>SNAMWESKFVKEGLTFDDVLLVPAKSDVLPREVSVKTVLSESLQLNIPLISAGMDTVTEADMAIAMARQGGLGIIHKNMSIEQQAEQVDKVKRSGGLLVGAAVGVTADAMTRIDALVKASVDAIVLDTAHGHSQGVIDKVKEVRAKYPSLNIIAGNVATAEATKALIEAGANVVKVGIGPGSICTTRVVAGVGVPQLTAVYDCATEARKHGIPVIADGGIKYSGDMVKALAAGAHVVMLGSMFAGVAESPGETEIYQGRQFKVYRGMGSVGAMEKGSKDRYFQEGNKKLVPEGIEGRVPYKGPLADTVHQLVGGLRAGMGYCGAQDLEFLRENAQFIRMSGAGLLESHP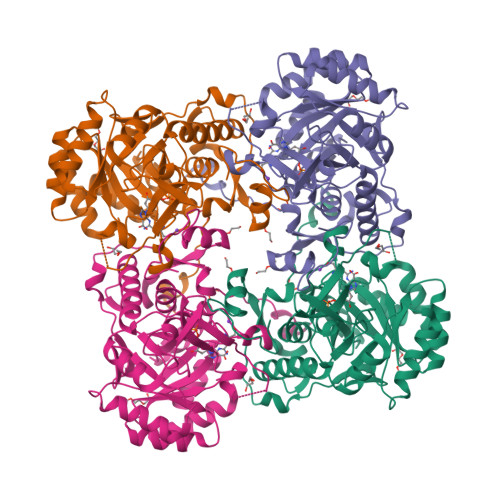HHVQITKEAPNYSL[2x]> MATVKTTHRTIAGWDGTPLGAFVIEPQ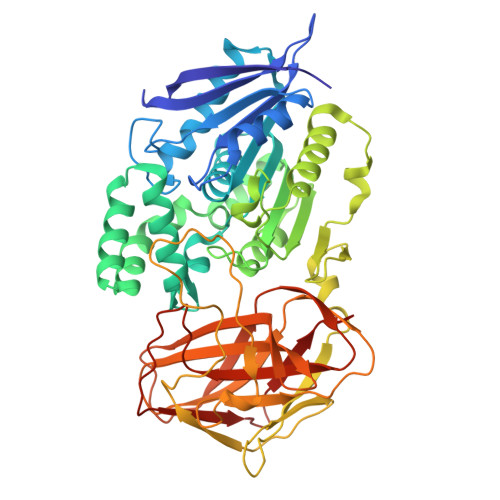DAGGGRYPLLVMPSSWAVPSVEYVGVAQSLAQRGYVVISYSSRGFWESGGSIDIAGPSTVEDVSALIDWALDNTRADPDRIGVSGISYGAGTSLLAAARDPRIKAVAALSGWADLQASLYSNDTPSAQGIALLVAAGLVTGRPGAELATINRNVLAGNYQGAVDSLLPVAAQRSPAASIDEINANQPAVFLANAFNDSLFPPGQLVDFFNRLKGPKQLQLRHGDHALNEALGALGIPNEVYDQVGDWFDHYLKAVANGIDRQPAVQLKSQKGSWSSYPDWQATSKGAVSYGLTAPSGLLLPTGGLAEHGGGTGWNYRIGSGLLTAANSGVAMASGALQMINLPPGAYVPFVGRSAAGVWQGPIQWSAKRLDGAPEVRLTVTPSRANTTLYAYLYAEDVLGNGQLISHKPYTLRGATPGQAKTLDLRLEASSWNLPAGSRLTLVVDTVDLRYAGISQLGGAVTFTSPANAPSVLKVPLH The heterogeneous nuclear ribonuclearprotein, Nab2, a conserved Zn finger protein, is essential for mRNA production and functions in polyadenylation, surveillance and the packaging leading to generation of export-competent mRNPs. nab2 mutants frequently generate hyperadenylation, defects in surveillance, and reduced mRNA nuclear export resulting in nuclear accumulation of poly(A)-mRNA, but the impact on each of these functions often varies between mutants, consistent with the Nab2 protein having several functions in the gene expression pathway. The S. cerevisiae Nab2 protein contains four domains: an N-terminal PWI-like domain that interacts with NPCs, followed by a Gln-rich linker; an Arg-Gly (RGG) domain required for nuclear import; and finally a domain containing seven tandem CCCH Zn fingers that binds polyadenosine-RNA in vitro, contributes to poly(A) tail length control, and also functions as a checkpoint for proper 3΄ processing. The Zn finger domain is essential for Nab2 function and for its binding to poly(A) mRNA, albeit only fingers 5–7 are necessary and are sufficient for high affinity polyadenosine–RNA binding. Nab2 functions in this process to control both mRNP compaction that facilitates movement through nuclear pore complexes and the length of transcript poly(A) tails.

Crystals with P21 symmetry that diffracted to 1.55 Å resolution were obtained for the complex of A11G RNA with ZnF567. The asymmetric unit contained two heterotetramers that each contained two RNA and two protein chains. Within a heterotetrameter, each of the two RNA chains bound to both protein chains through interactions that were dominated by the purine rings of five of the bases being buried in surface cavities. In each protein chain, finger 5 bound to A4 and finger 7 bound to A5 and A6 of one RNA chain, whereas finger 6 bound to A10 and A11 of the other RNA chain. The 3΄ G12 did not interact directly with either protein chain, but appeared to contribute to the looping of the second half of the RNA chain that positioned A10 and A11 to facilitate interaction with finger 6. ZnF567 dimerization was mediated primarily by each RNA chain binding to two protein chains in an arrangement that was facilitated by the specific spatial arrangement of the three fingers so that the polyribonucleotide bound to fingers 5 and 7 of one chain and finger 6 of the other. With A4, A6 and A11, a H-bond between Adenine N6 and the SG of a cysteine in the finger was supplemented by the purine stacking on one side against an aromatic side chain while its other face formed putative π interactions with a positively-charged residue. Although the second binding geometry also stacked the purine of A5 and A10 against an aromatic side chain and formed π interactions, N6 instead formed a H-bond with a main chain carbonyl. In both cases, the H-bonds required the N6 hydrogens and so could not be formed by guanine O6, accounting for the specific recognition of adenosine by the fingers.

>GSEKSLEQCKFGTHCTNKRCKYRHARSHIMCREGANCTRIDCLFGHPINEDCRFGVNCKNIYCLFRHPPGRVLPEKK[4x]Phosphatidylinositol 3-kinase type 2α (PI3KC2α) and related class II PI3K isoforms are of increasing biomedical interest because of their crucial roles in endocytic membrane dynamics, cell division and signaling, angiogenesis, and platelet morphology and function. Class II PI3Ks comprise PI3KC2α, PI3KC2β and PI3KC2γ isoforms and are unique in their ability to directly synthesize PI 3,4-bisphosphate (PI(3,4)P2) from PI 4-monophosphate (PI(4)P) in vivo. PI3KC2α contains a compact PI3K catalytic core (PI3KC2αcore) that comprises a Ras-binding domain and an N-terminal C2 domain as well as helical and kinase domains and displays a typical PI3K kinase domain fold. The ATP-binding site of the unliganded apo form of PI3KC2αcore is located in a cavity between the N- and C-lobes of the kinase domain and encompasses the (1) adenine-binding pocket, (2) affinity pocket and (3) specificity pocket.

To explore the structural basis of the inhibitory mechanism of PITCOIN1–PITCOIN3, we determined the structures of PI3KC2αcore in complex with inhibitors at maximal resolutions ranging from 2.5 to 2.9 Å. PITCOINs adopt nearly identical positions in the ATP-binding site. Their pteridinone scaffold occupies the adenine-binding pocket, while the two vicinal (R1 and R2) arms that extend outward from the pteridinone moiety display specific interactions with the N-lobe of the kinase domain and cause the inhibitors to adopt a propeller-shaped conformation. The pteridinone scaffold of PITCOIN1–PITCOIN3 forms a single hydrogen bond with the backbone of V1187 located in the kinase hinge region and embeds into hydrophobic surfaces provided by M1136 and L1186 at the top, M1257 and I1267 at the bottom, and F1172 on the inside of the adenine-binding pocket. PITCOIN2 and PITCOIN3 are distinguished from PITCOIN1 by the presence of bulky hydroxyphenyl (that is, PITCOIN2) or N-phenylmethanesulfonamide (that is, PITCOIN3) substituents on the 4′ position of the thiazole group. The space demand of these polar and bulky groups leads to additional hydrophobic interaction between P1188 within the kinase hinge and the phenyl group on the R1 arm of PITCOIN2 and PITCOIN3. As a result of these alterations, the mild off-target activity of PITCOIN1 against PI3KC2γ is lost in PITCOIN2 and PITCOIN3. Interestingly, the terminal hydroxyphenyl and N-phenylmethanesulfonamide groups cause the respective phenyl moiety to adopt different orientations upon complex formation of PITCOIN2 and PITCOIN3 with PI3KC2α. The hydroxyphenyl group of PITCOIN2 faces inward and is stabilized through interaction with the solvent, whereas the N-phenylmethanesulfonamide group of PITCOIN3 forms hydrophobic interactions with E1131. While PITCOIN1 was found to be a moderate PI3KC2γ and PI3KC2β inhibitor with IC50 values of about 1 µM or above, PITCOIN2 exhibited selectivity against PI3KC2γ but showed micromolar activity on PI3KC2β.

> GAVQNDEVAAFCQSIMKLKTKFPYTDHCTNPGYLLSPVTVQRNMCGENASVKVSIEIEGLQLPVTFTCDVSSTVEIIIMQALCWVHDDLNQVDVGSYILKVCGQEEVLQNNHCLGSHEHIQNCRKWDTEIKLQLLTLSAMCQNLARTAEDDEAPVDLNGSGSVMTRHSAGAGSGASTGCPRGSRNIKEAWTATEQLQFTVYAAHGISSNWVSNYEKYYLICSLSHNGKDLFKPIQSKKVGTYKNAAYLIKWDELIIFPIQISQLPLESVLHLTLFGVLNQSSGSSPDSNKQRKGPEALGKVSLTLFDFKRFLTCGTKLAYLWTSSHTNSIPGAIPKKSYVMERIVLQVDFPSPAFDIIYTSPQIDRNIIQQDKLETLESDIKGKLLDIIHRDSSFGLSKEDKVFLWENRYYCLKHPNCLPKILASAPNWKWANLAKTYSLLHQWPPLCPLAALELLDAKFADQEVRSLAVSWMEAISDDELADLLPQFVQALKYEIYLNSSLVRFLLSRALGNIQIAHSLYWLLKDALHDTHFGSRYEHVLGALLSVGGKGLREELSKQMKLVQLLGGVAEKVRQASGSTRQVVLQKSMERVQSFFLRNKCRLPLKPSLVAKELNIKSCSFFSSNAMPLKVTMVNADPLGEEINVMFKVGEDLRQDMLALQMIKIMDKIWLKEGLDLRMVIFRCLSTGRDRGMVELVPASDTLRKIQVEYGVTGSFKDKPLAEWLRKYNPSEEEYEKASENFIYSCAGCCVATYVLGICDRHNDNIMLRSTGHMFHIDFGKFLGHAQMFGSFKRDRAPFVLTSDMAYVINGGEKPTIRFQLFVDLCCQAYNLIRKQTNLFLNLLSLMIPSGLPELTSIQDLKYVRDALQPQTTDAEATIFFTRLIESSLGSIATKFNFFIHNLAQLRFSG>MPRPGHIAMVSVPSRGHLHPSLELIRELVARGHRVTYANDPSVAAAVTETGAELVPYTSALPSTDTTEGRVTDQIAQMDVFLDDAVGMLPQLRAAYEEDRPDVFLYDVLAYPARVLAMNWGIPSIQISPTWVMPEKYRERMAPVVEQLKQDPRGAAHYRRFDAWLEDSGVPGIDAGDLVNLPERSLVLVPRFLQPDADDVDEKRFTFIGPCLGRRAHQGDWKRPAGAEKVALVSLGSHLTNQLPFYETCVEVFAALPDWHLVLQIGRHVDAGELGELPPNVEVHNWVPQLAVLEQADVFVTHGGMGGIQEGLFSGVPMVVAPQANDQPANAESVVGLGIARRIDIATVTPDRLRAAVVELASDPAVAERLSGLRRELRAHGGTMRAADLIERQLPA[4x];>[4x]XNVFVGGVL

The glycosyltransferase Kcn28, which is unique among all CCNP BGCs, was expected to transfer a glycosyl group onto either the terminal COOH (5 and 6) or OH group (9 and 10). The monomeric Kcn28 contains two Rossmann-like β/α/β domains. The N-terminal domain from residues 6–208 is a substrate binding domain consisting of seven parallel β-strands that are flanked by seven α-helices, while the C-terminal domain comprising residues 229–392 is a UDP-sugar binding domain with six parallel β-strands surrounded by seven α-helices. A glycosyltransferase with relatively broad substrate specificity transfers sugars to the newly generated OH/COOH group.

We further attempted to understand the structural basis of the Kcn28-catalyzed enzymatic reaction. Crystal structures of Kcn28 as a free enzyme and in a binary complex (with 9) were obtained at 2.50 and 2.24 Å resolution, respectively (Fig. 4A and B and Table S17†). The model of 9 was confidently built into well-defined electron densities. Superposition of free and complexed structures revealed a global conformational change. The substrate 9 is tightly encapsulated in four α-helices with an orientation directed by insertion of the macrocyclic peptide part into the cavity and exposure of the cinnamic acid portion to the UDP part. Specifically, the side chains of F81, V108, and L109 create a hydrophobic environment to accommodate the cinnamic moiety of 9. In addition, the side chain of W131 provides hydrophobic interaction with the Phe residue of the macrocyclic peptide. The side chains of Q74, Q77, Y137, Y158 and N180 provide hydrogen bond interactions with the macrocyclic peptide backbone. Site-directed mutagenesis of the above key residues revealed diminished or abolished enzyme activities (Fig. S13†), supporting their roles in substrate binding. Consistent with the hypothesis, the H17A mutant renders the enzyme inactive.> MKKIYKQISGALLMLTLILNITACSPESFTSPNEAGIPVVSDY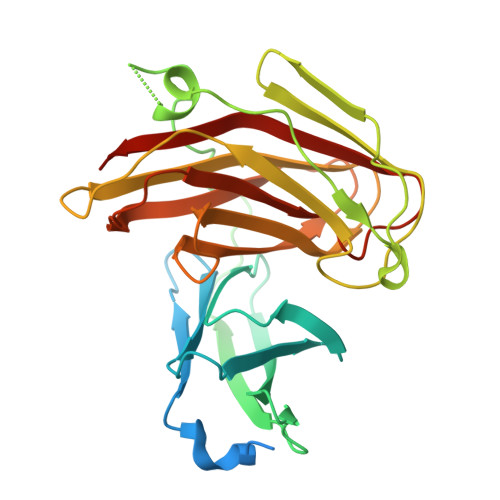EDCIRIDVNQETNYVTFSFQGQKGVMPIWIIDGKNYSSSFNMTKYYRKAGDYSVEVKIANSNGVSDRAITRNFHIDKTIMTGFGGFDPESNFNIWRTATISEPTFWYAPGWSQIADPAYSLVNGTYTVTLPEATSETWQAQMPIKTNIATDAGKNYDFSVILTSTIDHPNVTVKLVDATEDKIYYFEGKTPLVANEPVCFWKSNMPGLDIANLNLVFDFGGNAAGTVMTIESIVLKDHANDD> DQAGKSPAGVRYHGGDEIILQGFHWNVVREAPNDWYNILRQQASTIAADGFSAIWMPVPWRDFSSWSDGGKSGGGEGYFWHDFNKNGRYGSDAQLRQAAGALGGAGVKVLYDVVPNHMNRGYPDKEINLPAGQGFWRNDCADPGNYPNDCDDGDRFIGGESDLNTGHPQIYGMFRDELANLRSGYGAGGFRFDFVRGYAPERVDSWMSDSADSSFCVGELWKGPSEYPSWDWRNTASWQQII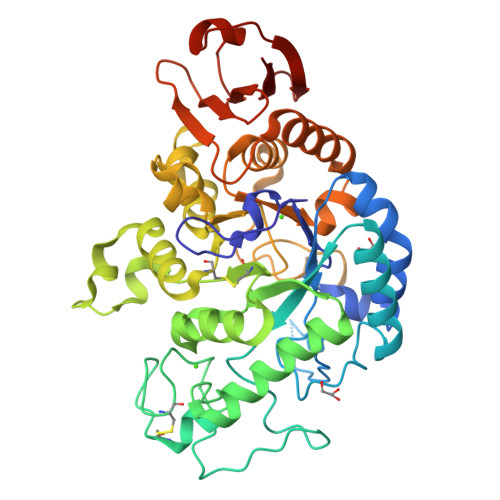KDWSDRAKCPVFDFALKERMQNGSVADWKHGLNGNPDPRWREVAVTFVDNHDTGYSPGQNGGQHHWALQDGLIRQAYAYILTSPGTPVVYWSHMYDWGYGDFIRQLIQVRRTAGVRADSAISFHSGYSGLVATVSGSQQTLVVALNSDLANPGQVASGSFSEAVNASNGQVRVWRS> GSHMTGGSVHSSPAIGQDGTIYVGSNDHYLYAINPNGKLKWKFET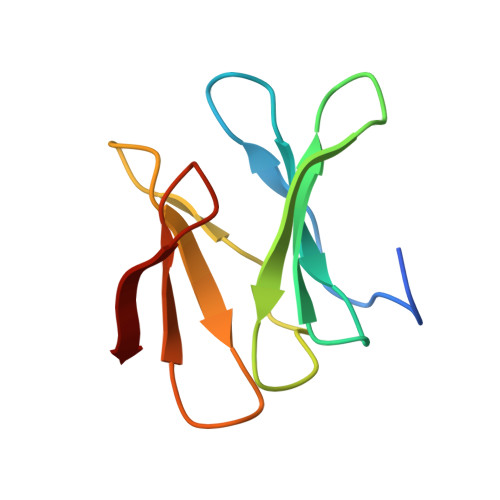GGSVHSSPAIGQDGTIYVGSNDHYLYAINPNGKLKWKFE>MAYFLDFDERALKEWRKLGSTVREQLKKKLVEVLESPRIEANKLRGMPDCYKIKLRSSGYRLVYQVIDEKVVVFVISVGKAERSEVYSEAVKRIL[2x]

The bacterial relBE locus encodes a toxin-antitoxin complex in which the toxin, RelE, is capable of cleaving mRNA in the ribosomal A site cotranslationally. The antitoxin, RelB, both binds and inhibits RelE, and regulates transcription through operator binding and conditional cooperativity controlled by RelE. Binding of RelB inhibits RelE by displacement of the C-terminal, flexible α-helix, which contains a tyrosine residue (Tyr87) that is critical for catalysis (Li et al., 2009). RelB is additionally known to dimerize through formation of a ribbon-helix-helix (RHH) DNA binding motif that allows transcriptional autoregulation through binding to the relO operator region (Li et al., 2008; Overgaard et al., 2009).

Two additional crystal structures of isolated RelE further show that the C-terminal helix uses this motif to adopt multiple, defined conformations. To better assess the structural rearrangements that take place in RelE upon RelB binding, we determined the structures of isolated RelE present in the two crystal forms obtained for the isolated toxin (P21 and P212121). In the structure of the P212121 crystal form, which has two molecules in the ASU, RelE also forms a domain-swap dimer involving the C-terminal helix; however, this interaction is not symmetrical. The interaction patterns observed between helix α3 and the core domain are identical in the RelE monomer, symmetrical dimer, and one molecule of the asymmetrical dimer, whereas they differ in the other molecule. The most common interaction is characterized by a strong salt bridge between Arg93 and Glu14 in addition to multiple contacts between hydrophobic residues such as Val86 and Tyr87 (left). In the alternative conformation observed in the asymmetrical dimer, the helix is pulled farther back and Arg93 now makes a hydrophobic interaction by stacking its guanidinium group on Phe74 (middle).>GAMGSMAKILCVLYDDPVDGYPKTYARDDLPKIDHYPGGQTLPTPKAIDFTPGQLLGSVSGELGLRKYLEANGHTFVVTSDKDGPDSVFEKELVDADVVISQPFWPAYLTPERIAKAKNLKLALTAGIGSDHVDLQSAIDRGITVAEVTYCNSISVAEHVVMMILGLVRNYIPSHDWARKGGWNIADCVEHSYDLEGMTVGSVAAGRIGLAVLRRLAPFDVKLHYTDRHRLPEAVEKELGLVWHDTREDMYPHCDVVTLNVPLHPETEHMINDETLKLFKRGAYIVNTARGKLADRDAIVRAI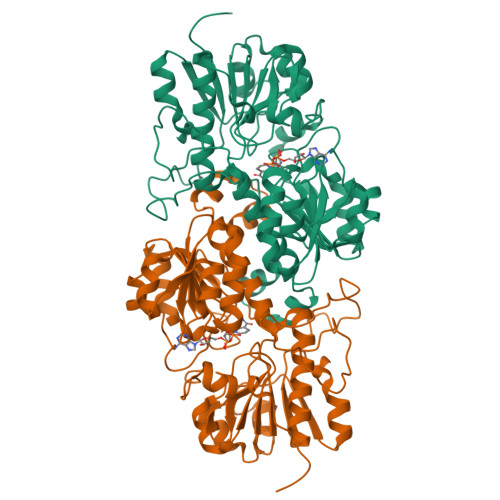ESGQLAGYAGDVWFPQPAPKDHPWRTMKWEGMTPHISGTSLSAQARYAAGTREILECFFEGRPIRDEYLIVQGGALAGTGAHSYSKGNATGGSEEAAKFKKAG[4x]>MRGHHHHHHGSGDLVAWNVKHDTRTLWTTPDTSPNCTIAQDKDSKLTLVLTKCGSQILANVSLIVVAGKYHIINNKNNPEIKSFTIKLLFDKNGVLLDNSNLGKTYWNFRSGDSNVSTAYEKAIGFMPNLVAYPKPSNSKKYARDIVYGTIYLGGKPDQPAVIKTT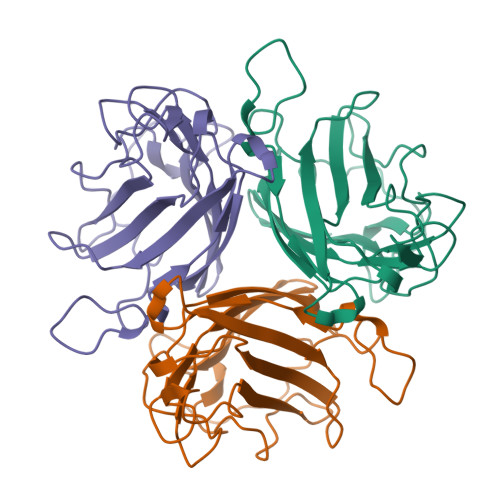FNQETGCEYSITFDFSWSKTYENVEFETTSFTFSYIAQQ[6x]N-(4-methoxyphenyl)glycinamide | C9 H12 N2 O2 | 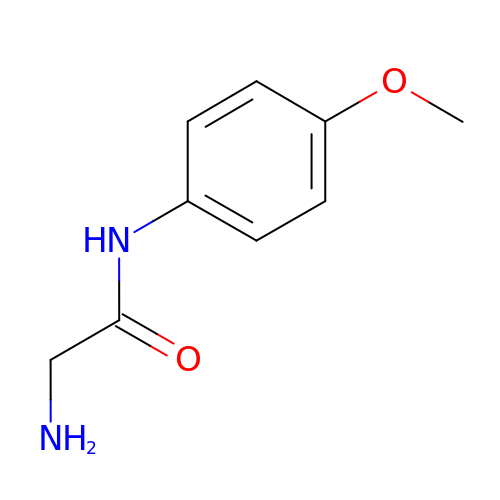MAVJTZKUNOKGPF-UHFFFAOYSA-N> GEIQWVKPNKETGRLNINGPTRTKLEPSVFHDVFEGNKEPAVLHSKDPRLEVDFEQALFSKYVGNTLYEPDEYIKEAALHYANQLKQLDIDTSQMSMEEACYGTENLEAIDLHTSAGYPYSALGIKKRDILDSTTRDVSKMKFYMDK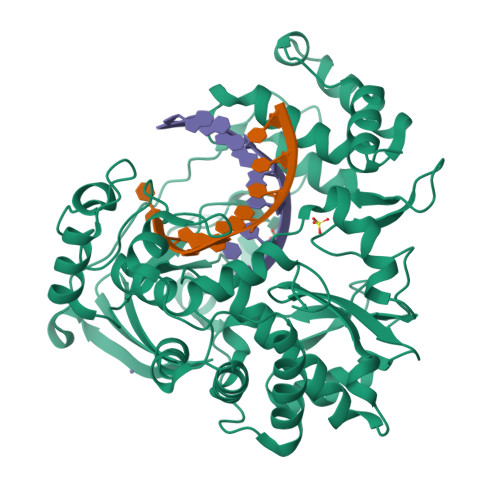YGLDLPYSTYVKDELRSIDKIKKGKSRLIEASSLNDSVYLRMTFGHLYETFHANPGTVTGSAVGCNPDTFWSKLPILLPGSLFAFDYSGYDASLSPVWFRALELVLREIGYSEEAVSLVEGINHTHHVYRNKTYCVLGGMPSGMSGTSIFNSMINNIIIRALLIKTFKGIDLDELNMVAYGDDVLASYPFPIDCLELARTGKEYGLTMTPADKSPCFNEVNWDNATFLKRGFLPDEQFPFLIHPTMPMKEIHESIRWTKDARNTQDHVRSLCLLAWHNGKQEYEKFVSAIRSVPVGKALAIPNYENLRRNWLELFHHHHHH> GSWQTYVDEHLMCEIEGHHLASAAILGHDGTVWAQSADFPQFKPEEITGIMKDFDEPGHLAPTGMFV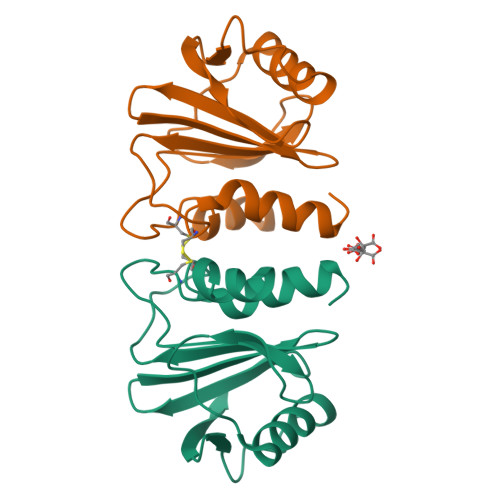AGAKYMVIQGEPGRVIRGKKGAGGITIKKTGQALVVGIYDEPMTPGQCNMVVERLGDYLVEQGM> VVGGLVALRGAHPYIAALYWGHSFCAGSLIAPCWVLTAAHCLQDRPAPEDLTVVLGQERRNHSCEPCQTLAVRSYRLHEAFSPVSYQHDLALLRLQEDADGSCALLSPYVQPVCLPSGAARPSETTLCQVAGWGHQFEGAEEYASFLQEAQVPFLSLERCSAPDVHGSSILPGMLCAGFLEGGTDACQGDSGGPLVCEDQAAERRLTLQGIISWGSGCGDRNKPGVYTDVAYYLAWIREHTV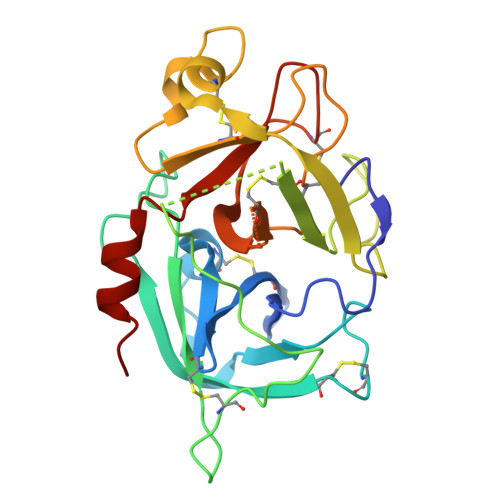S>[25x]T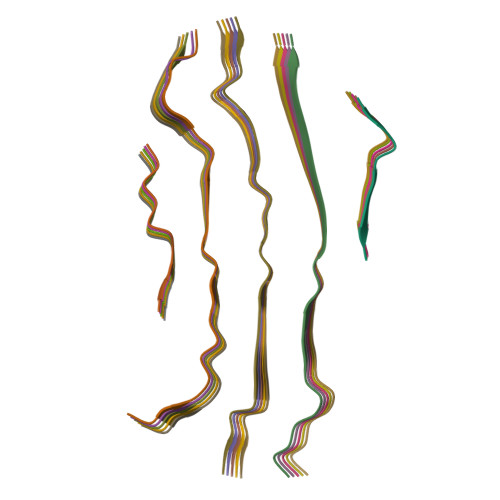GFSFGNTSTIGQPSTNTMGLFGVTQASQP>SMSSPQHPTPPARPRHMLGLPSTLFTPRSMESIEIDQKLQEIMKQTGYLTIGGQRYQAEINDLENLGEMGSGTCGQVWKMRFRKTGHVIAVKQMRRSGNKEENKRILMDLDVV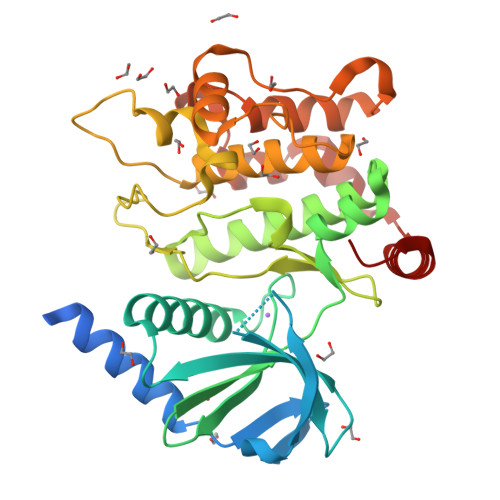LKSHDCPYIVQCFGTFITNTDVFIAMELMGTCAEKLKKRMQGPIPERILGKMTVAIVKALYYLKEKHGVIHRDVKPSNILLDERGQIKLCDFGISGRLVDDKAKDRSAGCAAYMAPERIDPPDPTKPDYDIRADVWSLGISLVELATGQFPYKNCKTDFEVLTKVLQEEPPLLPGHMGFSGDFQSFVKDCLTKDHRKRPKYNKLLEHSFIKRYETLEVDVASWFKDVMAKTESPR[3x]RecQ helicases, a family of DNA unwinding enzymes that are conserved from bacteria to mammals, play a key role in protecting the genome against deleterious changes (for recent reviews). Mutations in BLM and WRN are associated with the rare genetic diseases Bloom and Werner syndromes, respectively. BLM acts preferentially on recombination and repair intermediates containing HJs to promote efficient branch migration. Novel structural motifs found in the domain, such as the acidic β-wing, the BLM-insertion, and the C-term extended loop, may contribute cooperatively to the specialized functions of BLM in relation to HJ.

The structures of human BLM RQC complexed with a phosphate ion and an arsenate ion were determined at resolutions of 2.7 and 2.9 Å, respectively. The asymmetric unit of each crystal contains two RQC monomers (Mol-A and -B), which are bridged to each other by the ion (P1 or As1) shared at the interface. Since the BLM RQC domain binds to DNA in solution, we predicted that the phosphate ion P1 in the crystal structure might mimic one of the phosphate groups in the DNA substrate. As schematically represented in Figure 2c, P1 is bound by Mol-A and -B through nearly identical interactions, even though the two molecules are crystallographically independent of each other. The side chains of Ser1121 in both Mol-A and -B form hydrogen bonds with P1, while Arg1139 only in Mol-A forms a salt bridge with the ion; in Mol-B, Arg1139 is less close to P1 (5.3 Å), and instead a main-chain nitrogen of Lys1122 ligates the ion. The somewhat distorted binding symmetry between Mol-A and -B is due to the limited space within the interface, which only allows binding of a single phosphate ion. Interestingly, the position of P1 strikingly overlaps with one of the backbone phosphates of the 3′-strand DNA (yellow).

>[2x]GPLGSKTKDYKTRDVTDDVKSIVRFVQEHSSSQGMRNIKHVGPSGRFTMNMLVDIFLGSKSAKIQSGIFGKGSAYSRHNAERLFKKLILDKILDEDLYINANDQAIAYVMLGNKAQTVLNGNLKVDFMETENSSSVKKQKALVAKVS> MSIIIRVEDLRAVYLVREGTIKAADGISLDILENSVTAIVGESASGKSTIIEAMTKTLPPNGRILSGRVLYKGKDLLTMREEELRKIRWKEIALVPQAAQQSLNPTMKVIEHFKDTVEAHGVRWSHSELIEKASEKLRMVRLNPEAVLNSYPLQLSGGMKQRVLIALALLLDPVVLILDEPTSALDVLTQAHIIQLLKELKKMLKITLIFVTHDIAVAAELADKVAVIYGGNLVEYNSTFQIFKNPLHPYTRGLINSIMAVNADMSKVKPIP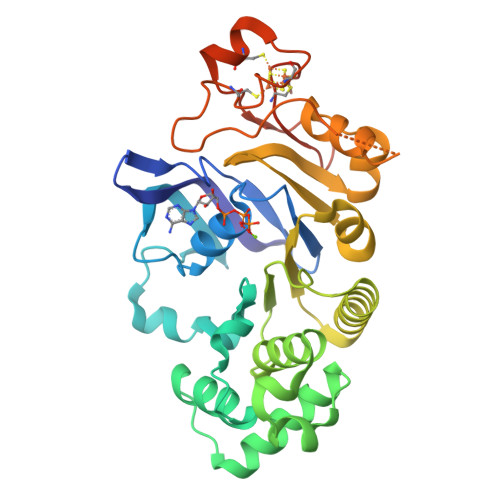GDPPSLLNPPSGCRFHPRCEYAMEICKKEKPKWIRLDGEAHVACHLYEEGRPLKLEHHHHHH> GAMGRILFLTTFMSKGNKVVRYLESLHHEVVICQEKVHAQSANLQEIDWIVSYAYGYILDKEIVSRFRGRIINLHPSLLPWNKGRDPVFWSVWDETPKGVTIHLIDEHVDTGDILVQEEIAFADEDTLLDCYNKANQAIEELFIREWENIVHGRIAPYRQTAGGTLHFKADRDFYKNLNMTTVRELLALKRLCAEPKRGEKPIDKTFHQLFEQQVEMTPDHVAVVDRGQSLTYKQLNERANQLAHHLRGKGVKPDDQVAIMLDKSLDMIVSILAVMKAGGAYVPIDPDYPGERIAYMLADSSAAILLTNALHEEKANGACDIIDVHDPDSYSENTNNLPHVNRPDDLVYVMYTSGSTGLAKGVMIEHHNLVNFCEWYRPYFGVTPADKALVYSSFSFDGSALDIFTHLLAGAALHIVPSERKYDLDALNDYCNQEGITISYLPTGAAEQFMQMDNQSFRVVITGGDVLKKIERNGTYKLYNGYGPTECTIMVTMFEVDKPYANIPIGKPIDRTRILILDEALALQPIGVAGELFIVGEGLGRGYLNRPELTAEKFIVHPQTGERMYRTGDRARFLPDGNIEFLGRLDNLVKIRGYRIEPGEIEPFLMNHPLIELTTVLAKEQADGRKYLVGYYVAPEEIPHGELREWLGNDLPDYMIPTYFVHMKAFPLTANGKVDRRALPDVQADAELLGEDYVAPTDELEQQLAQVWSHVLGIPQMGIDDHFLERGGDSIKVMQLIHQLKNIGLSLRYDQLFTHPTIRQLKRLLTEQKQVSLEPLRELDEQAEYETSAVEKRMYIIQQQDVESIAYNVVYTINFPLTVDTEQIRVALEQLVLRHEGLRSTYHMRGDEIVKRIVPRAELSFVRQTGEEESVQSLLAEQIKPFDLAKAPLLRAGVIETADKKVLWFDSHHILLDGLSKSILARELQALLGQQVLSPVEKTYKSFARWQNEWFASDEYEQQIAYWKTLLQGELPAVQLPTKKRPPQLTFDGAIQMYRVNPEITRKLKATAAKHDLTLYMLMLTIVSIWLSKMNSDSNQVILGTVTDGRQHPDTRELLGMFVNTLPLLLSIDHEESFLHNLQQVKAKLLPALQNQYVPFDKILEAARVKREGNRHPLFDVMFMMQGAPETELESNMHHINAGISKFDLTLEVLERENGLNIVFEYNTHLFD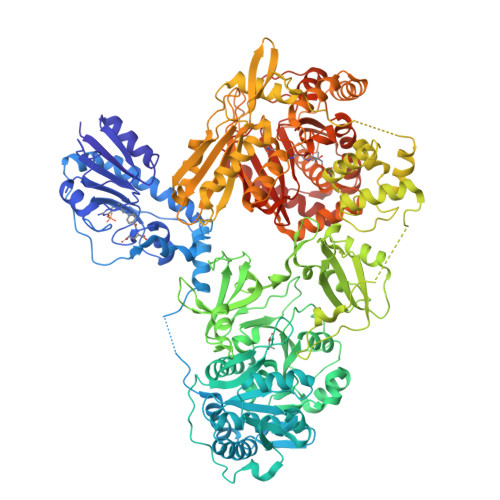EGMILRMVAQFEHLLLQAVHGLDQQVKRFELVAAAENLYFQ> MGHHHHHHSHMRTLAVISAGLSTPSSTRQIADSISEAVTAAVSARGEALS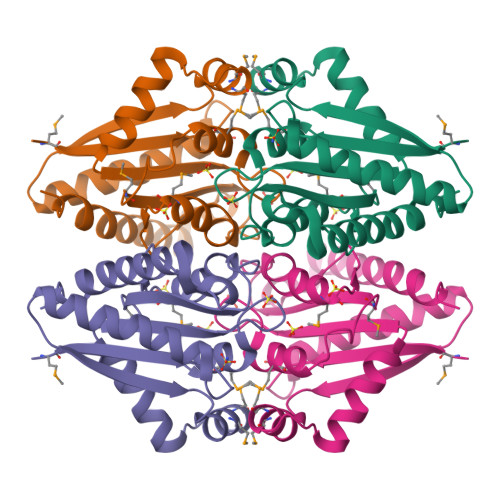VSTIELSELIPDLMTAMTTRVHTTKLEEITSALSASDGLVVATPVFKASYTGLFKMFFDILDTDALTGMPTIIAATAGSARHSLVLDYALRPLLSYMRAVVVPTGVFAATEDFGGPEGAEFNKRIARAAGELASLIVEESG(2R,3R,4S,5R)-2-({[(1R)-2-HYDROXY-1-PHENYLETHYL]AMINO}METHYL)-5-METHYLPYRROLIDINE-3,4-DIOL 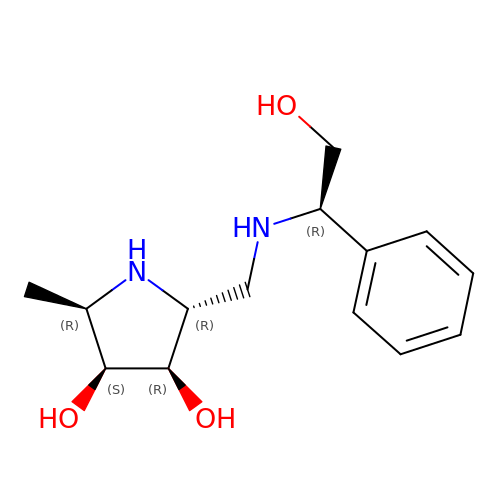| C14 H22 N2 O3 | KHLOMLBNZUMIHX-QKGWFMCXSA-N> MKTTTPLVHVASVEKGRSYEDFQKVYNAIALKLREDDEYDNYIGYGPVLVRLAWHISGTWDKHDNTGGSYGGTYRFKKEFNDPSNAGLQNGFKFLEPIHKEFPWISSGDLFSLGGVTAVQEMQGPKIPWRCGRVDTPEDTTPDNGRLPDADKDAGYVRTFFQRL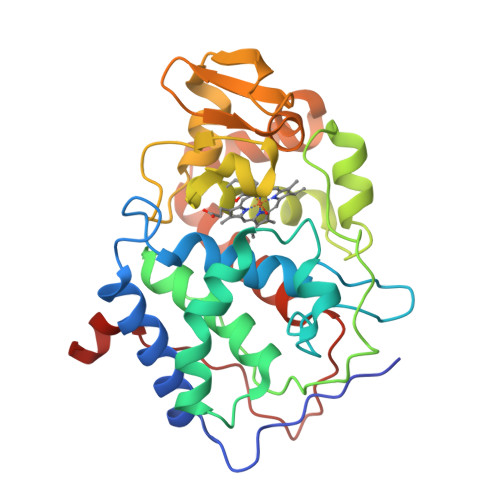NMNDREVVALMGAHALGKTHLKNSGYEGPWGAANNVFTNEFYLNLLNEDWKLEKNDANNEQWDSKSGYMMLPTAYSLIQDPKYLSIVKEYANDQDKFFKDFSKAFEKLLENGITFPKDAPSPFIFKTLEEQGL(2-[2-KETOPROPYLTHIO]ETHANESULFONATE 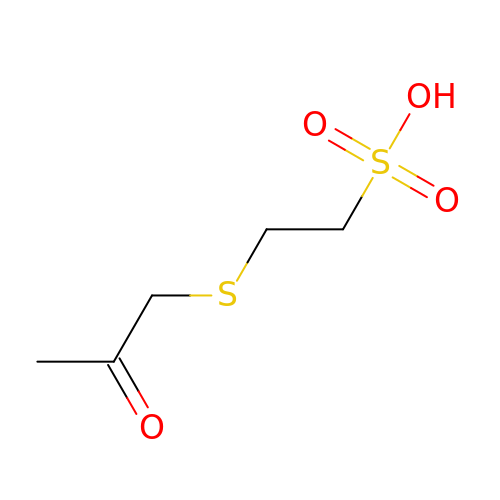| C5 H10 O4 S2 | CRNXHFXAXBWIRH-UHFFFAOYSA-N> MAHHHHHHMNPHPVEPRDQIAELLVESP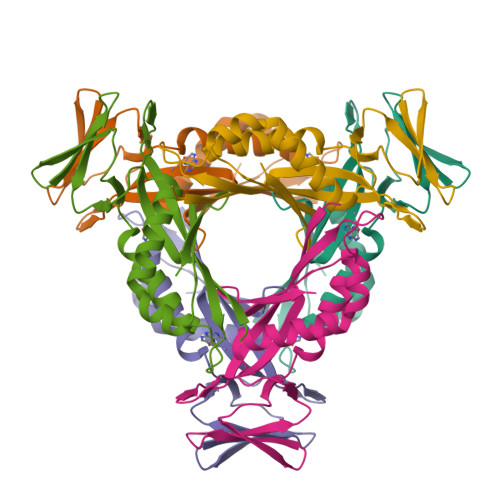LFSFNCAHFIAFKGFRETLHGHNYNVSLRLRGNIQGDGYVIDFSILKEKVRKVCKQLDHHFILPMYSDVLNIQEVNDNFKITCEDNSEYSFPKRDCVQIPIKHSSTEEIGLYILNQLIEEIDLPFLKTRSVNYMEVTVSESPSQKATVHRNI(1-HYDROXYHEPTANE-1,1-DIYL)BIS(PHOSPHONIC ACID) | C7 H18 O7 P2 | 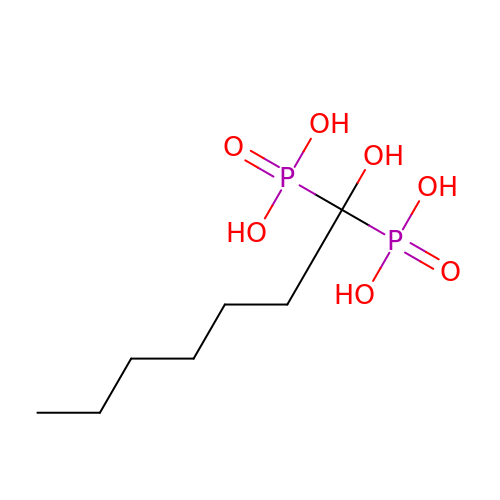IJEGNOYPWRBKAE-UHFFFAOYSA-N>[2x]LQALLPKAQSVGNSRVRFTTAEVDSAVARISQKIGVPASYYQFLIPIENFVVAGGFETTVSGSFRGLGQFNRQTWDGLRRLGRNLPAFEEGSAQLNASLYAIGFLYLENKRAYEASFKGRVFTHEIAYLYHNQGAPAAEQYLTSGRLVYPKQSEAAVAAVAAARNQHVKESWA

Lysins are lytic proteins that locally degrade the cell wall, either to provide access to the inner bacterial membrane during infection or to release virus progeny by cell lysis. P5ΔV8 adopts a lysozyme superfamily fold consisting of an N-terminal lobe (NTL) and a C-terminal lobe (CTL) connected by a central helix. The two lobes create a substrate binding cleft containing the predicted catalytic residue Glu95. However, in LTs, there is only one acidic residue, typically a glutamic acid, in the vicinity of the substrate cleavage site. Φ6 P5 adopts a lysozyme superfamily fold and our structure of P5 bound to a tetrasaccharide substrate analog shows that the enzyme contains a single glutamate (Glu95) in its active site. Together, our structural data unambiguously identify Φ6 P5 as an LT.

To understand the molecular basis of the thermostabilization of P5 by the V207F mutation we determined the crystal structures of P5ΔV8wt and P5ΔV8V207F at 1.4 Å resolution (we could not obtain crystals of P5wt or P5V207F). The structures of P5ΔV8wt and P5ΔV8V207F are almost identical, with a root mean square deviation (rmsd) of the Cα positions of 0.135 Å. Residue 207 is located on helix α8, facing the hydrophobic core of the protein. In P5ΔV8wt, V207 and adjacent residues 153, 176, 179–180, 194, 199, and 203–204 create a small (30.28 Å3) cavity lined with hydrophobic side chains. The lack of electron density within the cavity suggests that it is unoccupied. We note that P5ΔV8 forms an unusual crystal-packing interaction in which three N-terminal residues (residues 48–50) of one of the two subunits in the asymmetric unit insert into a shallow groove in a molecule in the adjacent asymmetric unit. Given that residues 48–50 make specific crystal contacts it was surprising that residues 53–59 were disordered and only residues 48–52 and 60–220 could be modeled. We will refer to the largest fragment, residues 48–220, as P5ΔV8.>[2x]ESTRNDVAWYARYPHILEEATRLPFAYPIGQYYDTGYSVASATEWSKYVDTSLTIPGVMCVNFTPTPGESYNKNSPINIAAQNVYTYVRHMNSGHANYEQADLMMYLLAMDSLYIFHSYVRKILAISKLYTPVNKYFPRALLVALGVDPEDVFANQAQWEYFVNMVAYRAGAFAAPASMTYYERHAWMSNGLYVDQDVTRAQIYMFKPTMLWKYENLGTTGTKLVPLMMPKAGDNRKLVDFQVLFNNLVSTMLGDEDFGIMSGDVFKAFGADGLVKLLAVDSTTMTLPTYDPLILAQIHSARAVGAPILETSTLTGFPGRQWQITQNPDVNNGAIIFHPSFGYDGQDHEELSFRAMCSNMILNLPGEAHSAEMIIEATRLATMFQVKAVPAGDTSKPVLYLPNGFGTEVVNDYTMISVDKATPHDLTIHTFFNNILVPNAKENYVANLEL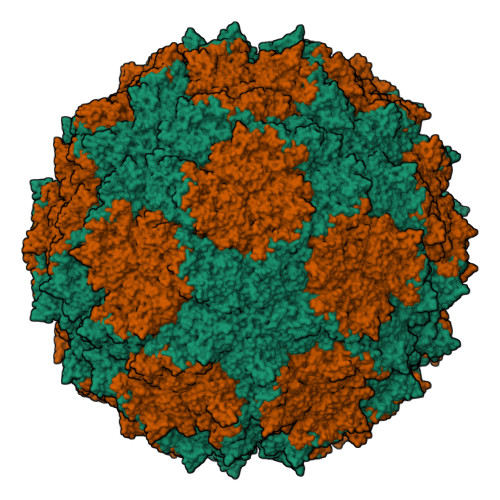LNNIIQFDWAPQLYLTYGIAQESFGPFAQLNDWTILTGETLARMHEVCVTSMFDVPQMGFNK> GSHMQNNSAKQSWLLRLFESKLFDISMAISYLYNSKEPGVQAYIGNRLFCFRNEDVDFYLPQLLNMYIHMDEDVGDAIKPYIVHRCRQSINFSLQCALLLGAYSSDMHISTQRHSRGTKLRKLILSDELKPANLKRTAANPKVENEDEPVRLAPEREFIKSLMAIGKRLATLPTKEQKTQRLISELSLLNHKLPARVWLPTAGFDHHVVRVPHTQAVVLNSKDKAPYLIYVEVLECENFDTTSVPARIPENRRDPEDPSAVALKEPWQEKVRRIREGSPYGHLPNWRLLSVIVKCGDDLRQELLAFQVLKQLQSIWEQERVPLWIKPYKILVISADSGMIEPVVNAVSIHQVKKQSQLSLLDYFL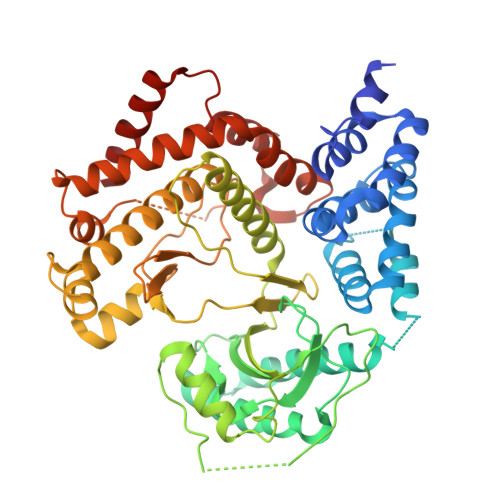QEHGSYTTEAFLSAQRNFVQSCAGYCLVCYLLQVKDRHNGNILLDAEGHIIHIDFGFILSSSPRNLGFETSAFKLTTEFVDVMGGLDGDMFNYYKMLMLQGLIAARKHMDKVVQIVEIMQQGSQLPCFHGSSTIRNLKERFHMSMTEEQLQLLVEQMVDGSMRS pyrimidin-5-amine | C4 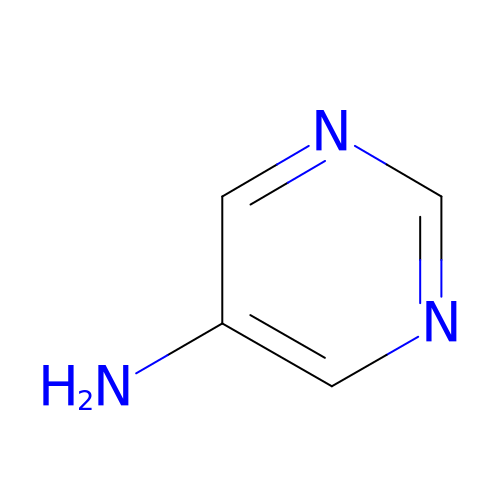H5 N3 | FVLAYJRLBLHIPV-UHFFFAOYSA-N5-PHOSPHO-D-ARABINOHYDROXAMIC ACID | C5 H12 N O9 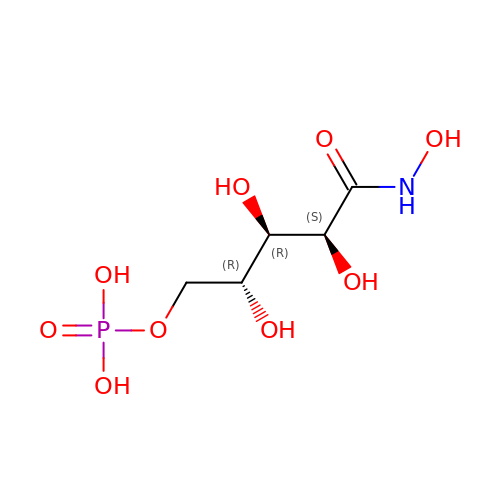P | OHQFMJPEBPCIEQ-JJYYJPOSSA-N RHODAMINE 6G | C28 H31 N2 O3 | 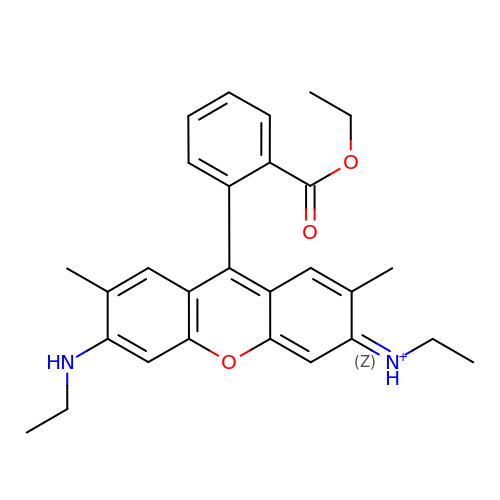IWWWBRIIGAXLCJ-KRUMMXJUSA-O>[4x]MLKAWHLPVAPFIKEQQERLMITLWLSGDDLPPRVTLRAEEDNEELSLPMHRLRQAPHPGVVAWRGEINLVNGQPRRRYSFKLLWADRQLWFTPQEFNRFPPARLEQFAVDLPDSGPQWVADQVFYQIFPDRFARSQSREAEQDATYYHHAAGHDIVRKAWDEPLTAEAGGSTFYGGDLDGISEKLPYLKQLGVTALYLNPVFVAPSVHKYDTEDYRRVDPQFGGDAALLRLRHNTQKEGMRLILDGVFNHSGDSHYRSSTLIDEIYGGEDSVVRHWLKAPWSMDGWRLDVVHMLGEGGGARNNLRHIAGITQAAKLERPDAFVFGEHFGDARQWLQADVEDSAMNYRGFTFPLWGFLANTDISYDPQKIDAQTCMAWMDNYRAGLSHQQQLRMFNQLDSHDTARFKSLLGKDVARLPLAVVWLFSWPGVPCI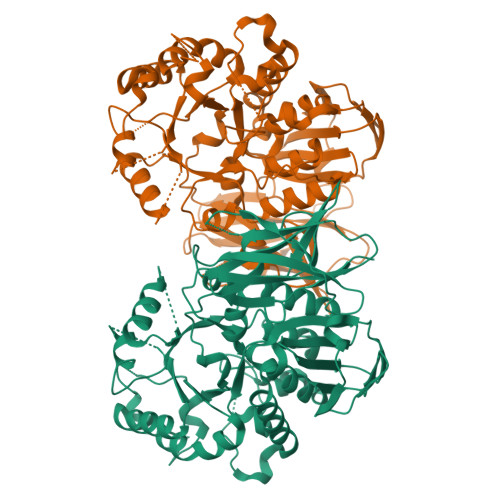YYGDEVGVDGNNDPFCRKPFPWDPALQDGDLLDLYKRMSKLRKAHQALRYGGCQVIYAEDNVVVFVRVYKQQRVLVAINRGEACEVVIEDSPLLDVNGWQLKEGAGALHDGVLTLPAISASVWFSR> MSNLLTVHQNLPALPVDATSDEVRKNLMDMFRARQVFSEHTWKMLLSVCRSWAAWCKLNNRKWFPAEPEDVRDYLLYLQARGLAVKTIQQHLGQLNMLHRRSGLPRPSDSNAVSLVMRRIRKENVDAGERAKQALAFERTDFDQVRSLMENSDRCQDIRNLAFLGI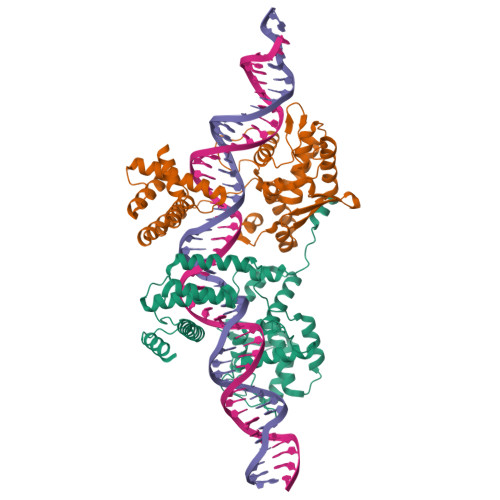AYNTLLRIAEIARIRVKDISRTDGGAMLIHIGRTKTLVSTAGVEKALSLGVTKLVERWISVSGVADDPNNYLFCRVRKNGVAAPSATSQLSTRALEGIFEATHRLIYGAKDDSGQRYLAWSGHSARVGAARDMARAGVSIPEIMQAGGWTNVNIVMNYIRNLDSETGAMVRLLEDGD;> MSNLLTVHQNLPALPVDATSDEVRKNLMDMFRDRQAFSEHTWKMLLSVCRSWAAWCKLNNRKWFPAEPEDVEDYLLYLQARGLAVKTIQQHLGQLNMLHRRSGLPRPSDSNAVSDVMRDIRKENVDAGERAKQALAFERTDFDQVRSLMENSDRCQDIRNLAFLGIAYNTLLRIAEIARIRVKDISRTDGGRMLIHIGRTKTLVSTAGVEKALSLGVTKLVERWISVSGVADDPNNYLFCRVRKNGVAAPSATSQLSTRALEGIFEATHRLIYGAKDDSGQRYLAWSGHSARVGAARDMARAGVSIPEIMQAGGWTNVNIVMNYIRNLDSETGAMVRLLEDGD>[60x]MNNLYRDLAPVTEAAWAEIELEAARTFKRHIAGRRVVDVSDPGGPVTAAVSTGRLIDVKAPTNGVIAHLRASKPLVRLRVPFTLSRNEIDDVERGSKDSDWEPVKEAAKKLAFVEDRTIFEGYSAASIEGIRSASSNPALTLPEDPREIPDVISQALSELRLAGVDGPYSVLLSADVYTKVSETSDHGYPIREHLNRLVDGDIIWAPAIDGAFVLTTRGGDFDLQLGTDVAIGYASHDTDTVRLYLQETLTFLCYTAEASVALSH

Encapsulins are a class of BMCs characterised by their conserved subunit (Enc), which self-assembles to encapsulate enzymatically active cargoes and can remain porous to cargo substrates. The overall structure of Enc subunits across species with different T numbers is conserved and consists of a peripheral domain (P-domain), an axial domain (A-domain), and an extension loop (E-loop). T = 1 encapsulins of Mycobacterium tuberculosis, the causative agent of tuberculosis, and the closely related Mycobacterium marinum, are known to encapsulate the DyP as a core cargo with iron storage ferritin protein (BfrB)28 and FolB as possible secondary cargoes. In vitro cryo-electron microscopy (EM) single-particle analysis of the Mycobacterium tuberculosis encapsulin was used to obtain three structures of the encapsulin shell in intermediate states, as well as a 2.3 Å structure of the fully assembled shell.

To study the structure of the encapsulin shell at near-atomic resolution, we overexpressed and isolated M. tuberculosis encapsulin from E. coli, which has 92.5% sequence identity (97% sequence similarity) with M. marinum. We used 89,072 particles which were found to be in the fully assembled state, yielding a 2.3 Å structure of the complete M. tuberculosis encapsulin shell. The encapsulin shell forms a T = 1 icosahedron and has an inner diameter of 19 nm and outer diameter of 23 nm, measured along a fivefold symmetry axis. The icosahedral assembly of 60 copies of Enctb can be described to consist of 12 pentamers, 20 trimers, or 30 dimers. The dimers are formed by the interaction of E-loops from Enctb subunits of two neighbouring faces, forming a tight interaction. The M. tuberculosis encapsulin shell has multiple different pores; single pores are present in the centres of each pentamer (9 Å diameter) and trimer (6 Å diameter) and two pores are present at the interface between two Enctb subunits within the pentamer (9 Å and 5 Å diameter). We did not find a clear pore at the points of twofold symmetry. The diameter of the central fivefold pore is relatively large compared to the reported pore size of other species, such as 6.8 Å in M. smegmatis, and 8 Å in M. hassiacum. Overall, the encapsulin shell structure of M. tuberculosis is similar to T = 1 from other species, with some species-specific variations, such as the relatively large fivefold pore diameter and the rotation of the distal section of the E-loop. A notable difference compared to M. hassiacum is the absence of a disulphide bridge between Cys134 and Cys254 in the M. tuberculosis encapsulin.> GSHTAEEDMEDDTSWRSEATFQFTVERFSRLSESVLSPPCFVRNLPWKIMVMPRFYPDRPHQKSVGFFLQCNAESDSTSWS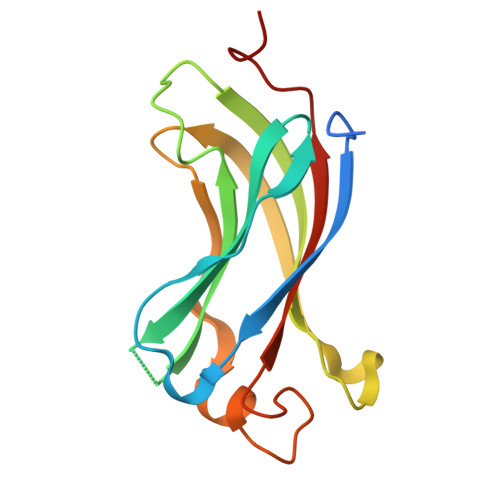CHAQAVLKIINYRDDEKSFSRRISHLFFHKENDWGFSNFMAWSEVTDPEKGFIDDDKVTFEVFVQADAPHGVAW> MGQEDPNSLRHKYNFIADVVEKIAPAVVHIELFRKLPFSKREVPVASGSGFIVSEDGLIVTNAHVVTNKHRVKVELKNGATYEAKIKDVDEKADIALIKIDHQGKLPVLLLG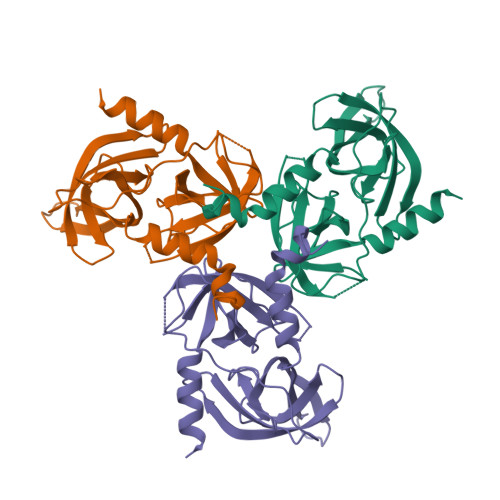RSSELRPGEFVVAIGSPFSLQNTVTTGIVSTTQRGGKELGLRNSDMDYIQTDAIINYGNAGGPLVNLDGEVIGINTLKVTAGISFAIPSDKIKKFLTESHDRQAKGKAITKKKYIGIRMMSLTSSKAKELKDRHRDFPDVISGAYIIEVIPDTPAEAGGLKENDVIISINGQSVVSANDVSDVIKRESTLNMVVRRGNEDIMITVIPEEIDPLEHHHHHH> QIGWRREGIKYRRNELFLDVLESVNLLMSPQGQVLSAHVSGRVVMKSYLSGMPECKFGMNDKIVIEXXXXXXXXXXXXXXXXXXXXXXXXXXXXXXXXXXXXXRSISFIPPDGEFELMRYRTTKDIILPFRVIPLVREVGRTKLEVKVVIKSNFKPSLLAQKIEVRIPTPLNTSGVQVICMKGKAKYKASENAIVWKIKRMAGMKESQISAEIELLPTNDKKKWARPPISMNFEVPFAPSGLKVRYLKVFEPKLNYSDHDVIKWVRYIGRSGIYETRC;> GYMPMSPG

Clathrin-mediated endocytosis (CME) is a major regulator of RTKs involving the heterotetrameric AP2 complex composed of large α and β2, medium μ2, and small σ2 subunits. AP2 binds to transmembrane cargo proteins that contain specific motifs such as YxxΦ (Y denotes Tyr; x, any amino acid; and Φ, bulky hydrophobic residue) serving as μ2 binding sites. In this study, we discovered AP2 is also an IRS-1-associated protein. IRS-1 binds with AP2 to prevent IGF-IR recruitment into clathrin-coated structures and thus enhance surface retention of activated IGF-IR.

We also analyzed the crystal structures of μ2 C-terminal subdomain (C-μ2) bound to IRS-1 YxxΦ motifs. Importantly, the side chains of Tyr and Met residues of IRS-1 YxxΦ motifs are inserted into the binding pockets of μ2, which are shared by the AP2 cargo proteins. Collectively, these results indicate that IRS-1 is recognized by the AP2 complex via the μ2 subunit in the very similar manner to conventional endocytic cargos. Using IRS-1 truncated mutants, we mapped the central region (amino acid residues 543–865) which is necessary for the binding to AP2. This region is almost identical to that for the clathrin adaptor AP1 complex found in our previous study, which binds to YxxΦ motifs of IRS-1 including Tyr 608, Tyr 628, and Tyr 658 via its μ1 subunit. Indeed, the Ala mutation of all these Tyr residues in IRS-1, but not a single substitution, completely abolished the binding to μ2 in vitro (IRS-1 3YA mutant). The Tyr residues of the YxxΦ motifs of IRS-1 (Tyr608, 628, and 658) critical for the binding to AP2 are part of phosphorylation sites among multiple Tyr residues in the C-terminus of IRS-1 that mediate the interaction of IRS-1 with PI3K and subsequent activation of PI3K. In addition, AP2 would preferentially bind non-phosphorylated IRS-1 since AP2 cannot recognize phosphorylated YxxΦ sequence due to its limited capacity. Our results indicate that IRS-1 inhibits the recruitment of IGF-IR to CCPs through YxxΦ motifs in IRS-1.>SNAMPMVAAVEFAKSPAEVLRVGSGFSLAGVDPESTPGYTGVKADGKALLAAQDARLAELQEKLFAEGKFGNPKRLLLILQAMDTAGKGGIVSHVVGAMDPQGVQLTAFKAPTDEEKSHDFLWRIEKQVPAAGMVGVFDRSQYEDVLIHRVHGWADAAELERRYAAINDFESRLTEQGTTIVKVMLNIS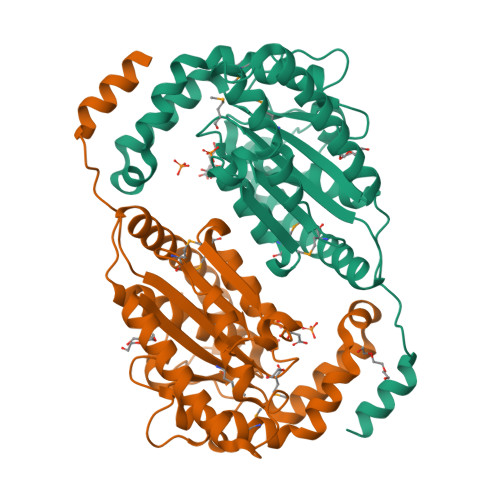KDEQKKRLIARLDDPSKHWKYSRGDLAERAYWDDYMDAYSVAFEKTSTEIAPWHVVPANKKWYARIAVQQLLLDALGGLQLDWPKADFDVAAERALVVES[4x]Filoviruses are unusual among mononegaviruses in that they encode an additional nucleocapsid component, VP30. VP30 is a multifunctional protein and acts as a transcriptional activator. The C-terminal domain of VP30 (CTD, amino acids 139–288) forms a conserved dimer of two globular, α-helical domains assembled by the extension of one α-helix from each protomer across the dimer interface to contact the adjacent protomer. Here, we have determined crystal structures and the biological functions of the protein complex formed by the filovirus transcriptional activator, VP30, and the core component of the nucleocapsid machinery, NP.

To overcome the low-affinity of the interaction, we expressed the EBOV NP peptide (600–627) as a fusion to the N terminus of EBOV VP30 CTD, and the MARV NP peptide (552–579) as a fusion to the N terminus of MARV VP30 CTD (146–281). The EBOV NP-VP30 fusion protein diffracted to 2.20 Å with ten protomers in the asymmetric unit, while the MARV NP-VP30 construct diffracted to 3.25 Å with eight protomers in the asymmetric unit. All of the EBOV NP peptides bind to VP30 in an identical fashion. Amino acids from the EBOV NP peptide contacting VP30 are primarily those that are highly conserved across ebolaviruses. NP contacts VP30 on the EBOV VP30 globular C-terminal domain, distal to the VP30 dimer interface. The NP-VP30 interface is primarily hydrophobic. Very few NP side chains make hydrogen bonds to VP30. However, NP R612 participates in a salt bridge to VP30 D202 and NP Y611 forms a hydrogen bond to VP30 E197. The NP peptide makes several hydrogen bonds using its main-chain atoms to the VP30 side chains of Q203, R213, Q229 and W230. The buried non-polar surface area calculated from the ITC experiments is 520 Å2, which is similar to the 620 Å2 of total buried surface area observed in the EBOV NP-VP30 crystal structure.

>[10x]MAHHHHHHVDDDDKMRTPTVAPPAPVYRDHSEKKELPQDEQQDGPKITLLTLIKTAEHWARQDIRTIEDSKLRALLTLCAVMTRKFSKSQLSLLCETHLRREGLGQDQAEPVLEVYQRLHSDKGGSFEAALWQQWDRQSLIMFITAFLNIALQLPCESSAVVVSGLRTLVPQSDNEEASTNPGTCSWSDEGTP> MGHHHHHHGEFKALTRRLQVEPRLLSKQMAGCLEDCTRQAPESPWEEQLARLLQEAPGKLSLDVEQAPSGQHSQAQLSGQQQRLLAFFKCCLLTDQLPLAHHLLVVHHGQRQKRKLLTLDMYNAVMLGWARQGAFKELVYVLFMVKDAGLTPDLLSYAAALQCMGRQDQDAGTIERCLEQMSQEGLKLQALFTAVLLSEEDRATVLKAVHKVKPTFSLPPQLPPPVNTSKLLRDVYAKDGRVSYPKLHLPLKTLQCLFEKQLHMELASRVCVVSVEKPTLPSKEVKHARKTLKTLRDQWEKALCRALRETKNRLEREVYEGRFSLYPFLCLLDEREVVRMLLQVLQALPAQGESFTTLARELSARTFSRHVVQRQRVSGQVQALQNHYRKYLCLLASDAEVPEPCLPRQYWEELGAPEALREQPWPLPVQMELGKLLAEMLVQATQMPCSLDKPHRSSRLVPVLYHVYSFRNVQQIGILKPHPAYVQLLEKAAEPTLTFEAVDVPMLCPPLPWTSPHSGAFLLSPTKLMRTVEGATQHQELLETCPPTALHGALDALTQLGNCAWRVNGRVLDLVLQLFQAKGCPQLGVPAPPSEAPQPPEAHLP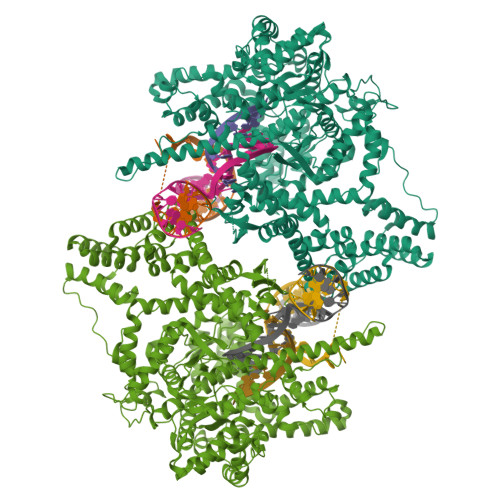HSAAPARKAELRRELAHCQKVAREMHSLRAEALYRLSLAQHLRDRVFWLPHNMDFRGRTYPCPPHFNHLGSDVARALLEFAQGRPLGPHGLDWLKIHLVNLTGLKKREPLRKRLAFAEEVMDDILDSADQPLTGRKWWMGAEEPWQTLACCMEVANAVRASDPAAYVSHLPVHQDGSCNGLQHYAALGRDSVGAASVNLEPSDVPQDVYSGVAAQVEVFRRQDAQRGMRVAQVLEGFITRKVVKQTVMTVVYGVTRYGGRLQIEKRLRELSDFPQEFVWEASHYLVRQVFKSLQEMFSGTRAIQHWLTESARLISHMGSVVEWVTPLGVPVIQPYRLDSKVKQIGGGIQSITYTHNGDISRKPNTRKQKNGFPPNFIHSLDSSHMMLTALHCYRKGLTFVSVHDCYWTHAADVSVMNQVCREQFVRLHSEPILQDLSRFLVKRFCSEPQKILEASQLKETLQAVPKPGAFDLEQVKRSTYFFS>MLGAVEGPRWKQAEDIRDIYDFRDVLGTGAFSE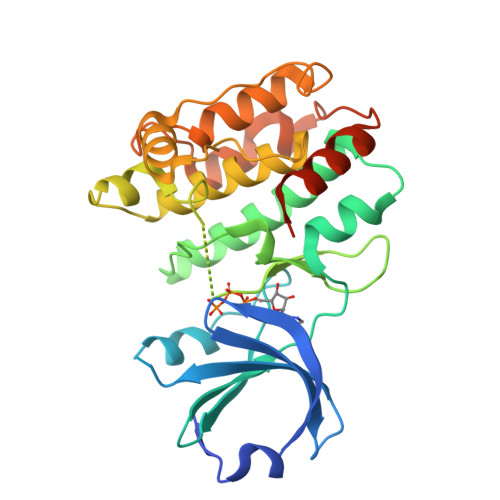VILAEDKRTQKLVAIKCIAKEALEGKEGSMENEIAVLHKIKHPNIVALDDIYESGGHLYLIMQLVSGGELFDRIVEKGFYTERDASRLIFQVLDAVKYLHDLGIVHRDLKPENLLYYSLDEDSKIMISDFGLSKMEDPGSVLSTACGTPGYVAPEVLAQKPYSKAVDCWSIGVIAYILLCGYPPFYDENDAKLFEQILKAEYEFDSPYWDDISDSAKDFIRHLMEKDPEKRFTCEQALQHPWIAGDTALDKNIHQSVSEQIKKNFAKSKWKQAFNATAVVRH[2x]>AKTHSVETPYGSVTFTVYGTPKPKRPAILTYHDVGLNYKSCFQPLFQFEDMQEIIQNFVRVHVDAPGMEEGAPVFPLGYQYPSLDQLADMIPCVLQYLNFSTIIGVGVGAGAYILARYALNHPDT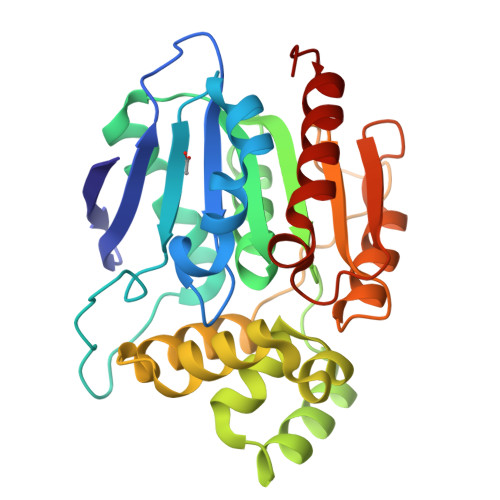VEGLVLINIDPNAKGWMDWAAHKLTGLTSSIPEMILGHLFSQEELSGNSELIQKYRNIITHAPNLDNIENYWNSYNNRRDLNFERGGDITLRCPVMLVVGDQAPHEDAVVECNSKLDPTQTSFLKMADSGGQPQLTQPGKLTEAFKYFLQGMGYMA[3x]> GAMEATPTPADLFSEDYLVDTLDGLTVDDQQAVLASLSFSKFLKHAKVRDWCAQAKIQPSMPALRMAYNYFLFSKVGEFIGSEDVCNFFVDRVFGGVRLLDVASVYAACSQMNAHQRHHICCLVERATSSQSLNPVWDALRDGIISSSKFHWAVKQQNTSKKIFSPWPITNNHFVAGPLAFGLRCEEVVKTLLATLLHPDETNCLDYGFMQSPQNGIFGVSLDFAANVKTDTEGRLQFDPNCKVYSIKCRFKYTFAKMECDPIYAA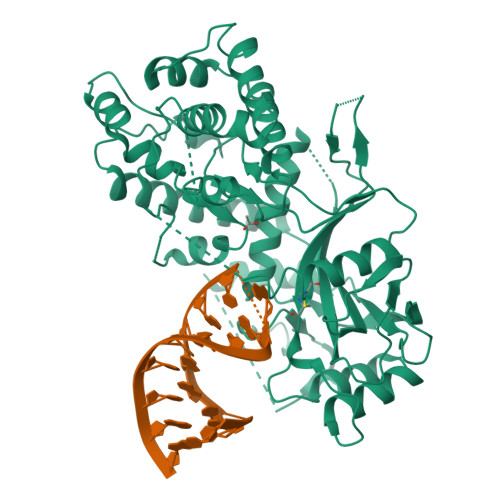YQRLYEAPGKLALKDFFYSISKPAVEYVGLGKLPSESDYLVAYDQEWEACPRKKRKLTPLHNLIRECILHNSTTESDVYVLTDPQDTRGQISIKARFKANLFVNVRHSYFYQVLLQSSIVEEYIGLDSGIPRLGSPKYYIATGFFRKRGYQDPVNCTIGGDALDPHVEIPTLLIVTPVYFPRGAKHRLLHQAANFWSRSAKDTFPYIKWDFSYLSANVPHSP>[4x]STKVVNVAVIGAGVVGSAFLDQLLAMKSTITYNLVLLAEAERSLISKDFSPLNVGSDWKAALAAS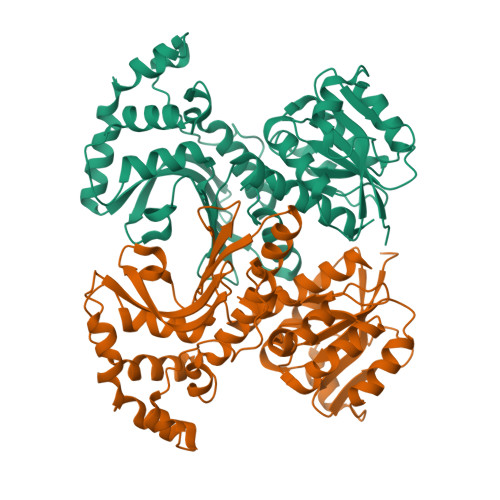TTKTLPLDDLIAHLKTSPKPVILVDNTSSAYIAGFYTKFVENGISIATPNKKAFSSDLATWKALFSNKPTNGFVYHEATVGAGLPIISFLREIIQTGDEVEKIEGIFSGTLSYIFNEFSTSQANDVKFSDVVKVAKKLGYTEPDPRDDLNGLDVARKVTIVGRISGVEVESPTSFPVQSLIPKPLESVKSADEFLEKLSDYDKDLTQLKKEAATENKVLRFIGKVDVATKSVSVGIEKYDYSHPFASLKGSDNVISIKTKRYTNPVVIQGAGAGAAVTAAGVLGDVIKIAQRL>MLYPEQNEARLKLSLDGTWAFALGSCAETQFDPAKPLPDAQPIAVPASYNDQNDQTTALRRHYGWVWYQRKVTLPAFCAGQRVVLRFGSVTHTAKVWLNGQLIAQHKGGFTPFEADVTALLQPGETALLTVACDNRVNHSTLPVGNEDGQLAFFGSDNAGIPSVEAAKRAAAPQNRPNFDFFNYAGIHRPVVLYTTPKEYIEDVTIVPAVDGTVQYAVKTTGSAPVRVTVLDADGNAVASAESAEGTITIPEVHLWEPRPGTPYLYTLHATCGADVYDQTFGVRSIEVRGTQVLLNGKPLYFKGFCKHEDFTAHGRGFDPVLNVKDVNLIHWANANAVRTSHYPYAEEFYDLCDREGILVMDETPAVGIGGGAAVNPYKEYPLAEHHRQVLAEMIHRDKNHPCVVLWSLGNEPNLEHFPQDAYDYWHPLYELAHQLDPQDRPVTLVCCQNDYTKDITTRTMDIVCINRYYGWYNLSGDMDAACYGLNQELDFWAEQHKPVMMSEYGADTVAGLHTAGAEMFSEEFQVEFYRRLDAEFDKRPWFVGEFVWNFADYDTVQGPMR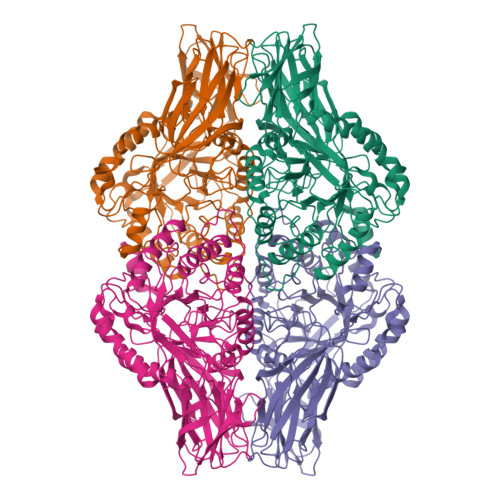VDGNKKGLFTRDRRPKLGMHFLRQRWAEIPTFGFK[4x]>[2x]MINTMTLDNGVRIITEKMSTVRSVSIGIWVGTGSRYESAEENGISHFLEHMFFKGTNTRSAQEIAEFFDSIGGQVNAFTSKEYTCYYAKVLDDHAGQAIDTLSDMFFHSTFQKEELEKERKVVFEEIKMVDDTPDDIVHDLLSSATYGKHSLGYPILG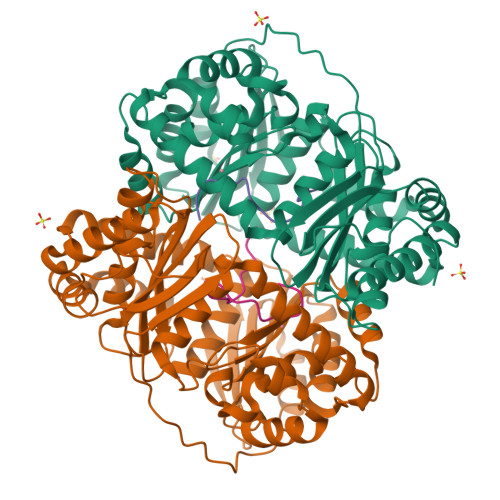TVETLNSFNEGMLRHYMDRFYTGDYVVISVAGNVHDELIDKIKETFSQVKPTTYNYQGEKPMFLPNRIVRKKETEQAHLCLGYPGLPIGDKDVYALVLLNNVLGGSMSSRLFQDIREKRGLCYSVFSYHSSFRDSGMLTIYAGTGHDQLDDLVYSIQETTSALAEKGLTEKELENGKEQLKGSLMLSLESTNSRMSRNGKNELLLKKHRSLDEMIEQINAVQKQDVSRLAKILLSASPSISLINANGELPKALIHLEHHHHHH;>AAAAAAAAAAAAAAAAA[2x]(2~{S},3~{S})-2-(fluoranylmethyl)-~{N}7-methyl-~{N}5-[(1~{R},5~{S})-3-oxabicyclo[3.1.0]hexan-6-yl]-3-phenyl-2,3-dihydro-1-benzofuran-5,7-dicarboxamide 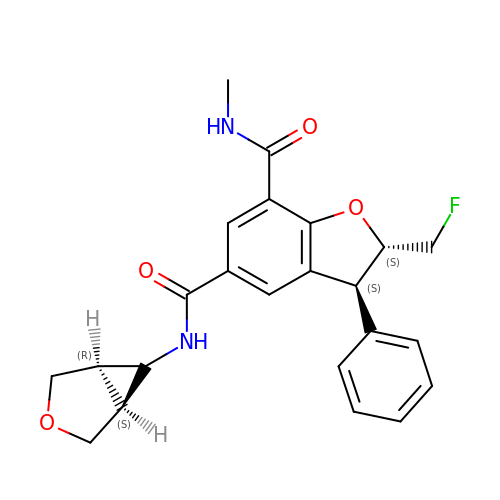| C23 H23 F N2 O4 | WZQLVEPIBAOOGF-RMMWZPCPSA-N>GPGSFKERRPFHERQKDVEEIRSQQPNKVPVIIERFDGERSLPLMDRCKFLVPEHITVAELMSIVRRRLQLHPQQAFFLLVNE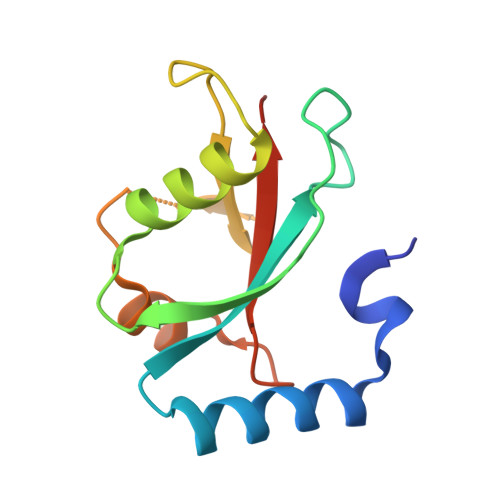RSMVSNSMSMSNLYSQERDPDGFVYMVYTSQPAFG[2x]>MASDYKDDDDKASDEVDAGTATMRGGALLCGQVQDEIEQLSRESSHFSLSTGILPSLGARSNRRVKLRRFVVSPYDHKYRIWEAFLVVLVVYTAWVSPFEFGFLRKPRPPLSITD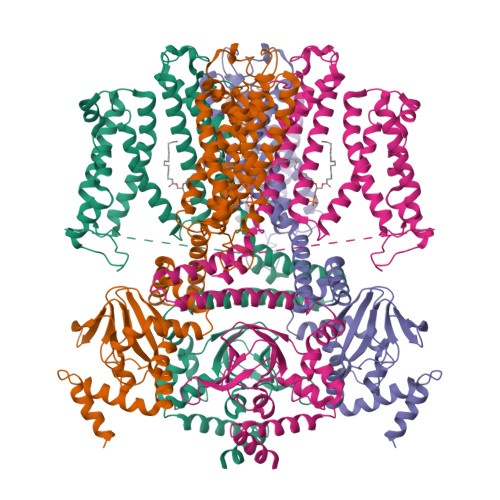NIVNAFFAIDIIMTFFVGYLDKSTYLIVDDRKQIAFKYLRSWFLLDLVSTIPSEAAMRISSQSYGLFNMLRLWRLRRVGALFARLEKDRNFNYFWVRCAKLVCVTLFAVHCAACFYYLIAARNSNPAKTWIGANVANFLEESLWMRYVTSMYWSITTLTTVGYGDLHPVNTKEMIFDIFYMLFNLGLTAYLIGNMTNLVVHGTSRTRNFRDTIQAASNFAHRNHLPPRLQDQMLAHLCLKYRTDSEGLQQQETLDALPKAIRSSISHFLFYSLMDKVYLFRGVSNDLLFQLVSEMKAEYFPPKEDVILQNEAPTDFYILVNGTADLVDVDTGTESIVREVKAGDIIGEIGVLCYRPQLFTVRTKRLCQLLRMNRTTFLNIIQANVGDGTIIMNNLLQHLKEMNDPVMTNVLLEIENMLARGKMDLPLNLCFAAIREDDLLLHQLLKRGLDPNESDNNGRTPLHIAASKGTLNCVLLLLEYHADPNCRDAEGSVPLWEAMVEGHEKVVKVLLEHGSTIDAGDVGHFACTAAEQGNLKLLKEIVLHGGDVTRPRATGTSALHTAVCEENIEMVKYLLEQGADVNKQDMHGWTPRDLAEQQGHEDIKALFREKLHERRVHIETSSSVPILKTGIRFLGRFTSEPNIRPASREVSFRIRETRARRKTNNFDNSLFGILANQSVPKNGLATVDEGRTGNPVRVTISCAEKDDIAGKLVLLPGSFKELLELGSNKFGIVATKVMNKDNNAEIDDVDVIRDGDHLIFATDS[4x]> GPASSNLIKQLQERGLVAQVTDEEALAERLAQGPIALYCGFDPTADSLHAGHLVPLLCLKRFQQAGHKPVALVGGATGLIGDPSFKAAERKLNTEETVQEWVDKIRKQVAPFLDFDCGENSAIAANNYDWFGNMNVLTFLRDIGKHFSVNQMINKEAVKQRLNREDQGISFTEFSYNLLQGYDFACLNKQYGVVLQIGGSDQWGNITSGIDLTRRLHQNQVFGLTVPLITKADGTKAGKTEGGAVWLDPKKTSPYKFYQFAINAADADVYRWLKFGTFMSIEEINALEEEDKNSGKAPRAQYVFAEQVTRLVHGEEGLQAAKRITECLFSGSLSALSEADFEQLAQDGVPMVEMEKGADLMQALVDSELQPSRGQARKTIASNAITINGEKQSDPEYFFKEEDRLFGRFTLLRRGKKNYCLICWK;> GPASSNLIKQLQERGLVAQVTDEEALAERLAQGPIALYCGFDPTADSLHAGHLVPLLCLKRFQQAGHKPVALVGGATGLIGDPSFKAAERKLNTEETVQEWVDKIRKQVAPFLDFDCGENSAIAANNYDWFGNMNVLTFLRDIGKHFSVNQMINKEAVKQRLNREDQG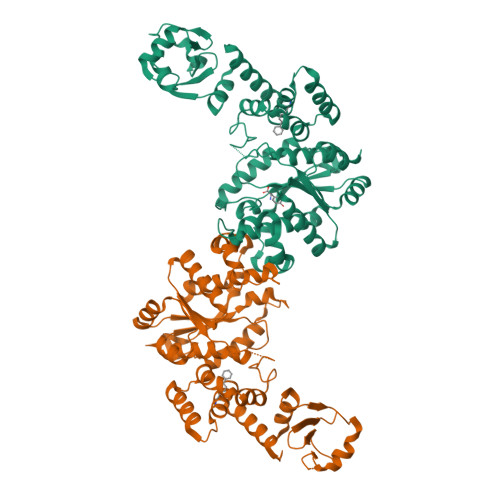ISFTEFSYNLLQGYDFACLNKQYGVVLQIGGSDQWGNITSGIDLTRRLHQNQVFGLTVPLITKADGTKAGKTEGGAVWLDPKKTSPYKFYQFAINAADADVYRWLKFGTFMSIEEINALEEEDKNSGKAPRAQYVFAEQVTRLVHGEEGLQAAKRITECLFSGSLSALSEADFEQLAQDGVPMVEMEXXXXXXXXXXXXXXXXXRLFGRFTLLRRGKKNYCLICWK(2R)-2,3-dihydroxypropyl beta-D-galactopyranoside | C9 H18 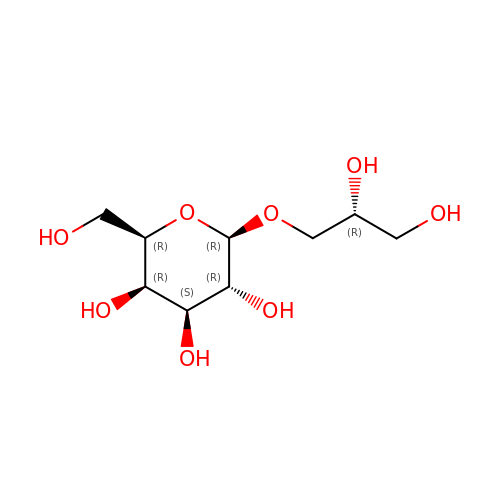O8 | NHJUPBDCSOGIKX-NTXXKDEISA-N>[2x]GMTRRIAICAPSTPFTREDSARVIALAAAEFPDLSLSFHEQCFASEGHFAGSDALRLSAFLECAN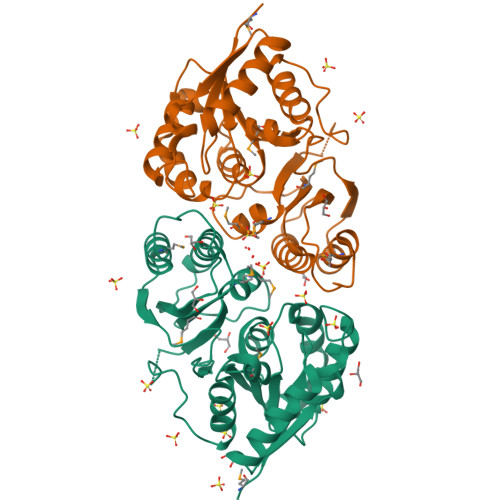DDAFEAVWFVRGGYGANRIAEDALARLGRAASAKQYLGYSDAGTLLAALYAHRIGRSVHAPMPVDIRRPEGESAVRRTLGWLAGAREGLEPTLGAGAPAVAFNLMTLAMLCGTRLLPDLSGHVVMIEEVAEHHYAVDRLLFHVTSCLADAGIAGLRLGRVSDVPENDRPFGCSVEEMARHWCHRAGIAFLGTADIGHDVDNRIVPFGLA Among them, cyanophage S-2L is unique because its genome has all its adenines (A) systematically replaced by 2-aminoadenines (Z). Here, we identify the enzyme that is responsible for genome duplication of the phage S-2L, a member of the PrimPol family, and we present its crystal structure. We confirm its polymerase activity but find that the enzyme is not specific to A or Z. Instead, we propose that the absence of A in S-2L genome is explained by a separate enzyme, an HD phosphohydrolase that specifically dephosphorylates dATP and that we name DatZ. We give a structural explanation for both the specificity and the reaction mechanism of DatZ, based on three crystallographic structures, including one determined at sub-angstrom resolution.

Each monomer of DatZ takes a globular form composed predominantly of α- and 310-helices (70% and 4% respectively), with no β-strands. The electron density allowed to build the whole protein as well as 218 water molecules around the DatZ chain (175 aa), which is roughly the number expected for this resolution limit. The base moiety of dA snugly fits in the catalytic pocket below a relatively flexible element (as indicated by higher B-factors), with the P79 residue on its tip. A catalytic divalent ion is found in the vicinity of dA’s free 5′-OH group, even though no divalent ion was added in buffers during purification or crystallisation. An excitation x-ray energy scan showed a major contribution of Zn; additionally, an anomalous double-difference signal at 40 sigmas at the Zn edge unambiguously point to the presence of a Zn2+ ion in this site. The fact that no additional divalent ions were added during protein purification indicates a high affinity of DatZ for Zn2+. In the catalytic site, the side chain of residue I22 is ideally positioned to sterically exclude the amino group in position 2 of the purine ring of G or Z and provides an immediate explanation for the observed specificity of the enzyme. Concerning the oligomeric state of DatZ, we found that in crystallo it arranges in a compact toroidal hexamer with a D3 symmetry, where neighbouring subunits are flipped. The whole hexamer is particularly rigid, as judged from the overall very low B-factors, which is consistent with the ultrahigh diffraction limit for DatZ crystals.

> GTGDGSMTLQITETYERLRASHISRWGIVQTTYPQNIAEHMWRVWLLCRDWGAAAGMPQHTVRQACEFALVHDLAEIRTGDAPTPHKTPELKELLAGIEAQIVPEVAELEATMAPEARELWKFCDTAEAVLFLKVNGLGAHAYDVQHLLMEQMKRRLMDSVLDVEVQDELMFQFERTIKKT>[2x]SNAACSKTNQNSKIATMKGDTITVADFYNEVKNSTASKQAVLSLLVSKVFEKQYGDKVSDKEVTKAYNEAAKYYGDSFSSALASRGYTKEDYKKQIRSEKLIEYAVKEEAKKEITDASYKSAYKDYKPEVTAQVIQLDSEDKAKSVLEEAKADGADFAKIAKDNTKGDKTEYSFDSGSTNLPSQVLSAALNLDKDGVSDVIKASDSTTYKPVYYIVKITKKTDKNADWKAYKKRLKEIIVSQKLNDSNFRNAVIGKAFKKANVKIKDKAFSEILSQY

Here, we solved the protein structures of two secreted parvulin and two secreted cyclophilin-like peptidyl-prolyl isomerase (PPIase) ATP-independent chaperones found in gram-positive streptococcal species. Two types of ATP-independent extracellular PPIases exist in pathogenic streptococci: the parvulin and cyclophilin families. Unlike cytoplasmic PPIases, extracellular PPIases have canonical secretion signal peptides that allow for their translocation across the cell membrane via the Sec pathway. These chaperones are lipidated to the outer leaflet of the membrane and function in the space between the bacterial membrane and cell wall.

Other streptococcal-secreted PPIases, such as S. mutans PrsA (SmuPrsA), are required for cell wall and membrane integrity and virulence in an infective endocarditis model. Additionally, the secretion of mutacin, the major factor in the colonization and establishment of S. mutans dental biofilms, is dependent on SmuPrsA. As key streptococcal virulence factors are dependent on PrsA for activity, we began characterizing streptococcal PrsA by determining the X-ray crystal structures of PrsA from S. pneumoniae and S. mutans. The SpnPrsA and SmuPrsA structures were solved to a resolution of 2.55 Å and 3.15 Å, respectively. As expected, SpnPrsA and SmuPrsA align well with an r.m.s.d. of 2.36 Å across 264 Cα atoms that share 49% sequence identity. Consistent with PrsA homologs, both streptococcal PrsA proteins have a central parvulin PPIase domain (SpnPrsA residues 143–241) linked to a foldase domain (N- and C-terminal regions). Furthermore, the streptococcal PrsA protomers are linked by a domain swap; protomers A and D each donate a segment of α1 and the β1, β2, and β7 strands to the domain swap. The interprotomer, three-stranded β-sheets formed by β1, β2, and β7 strands are presumed to interact with the cell membrane. Previous work of L. monocytogenes PrsA homologs has shown that dimerization is critical for PrsA function. This is consistent with our dimeric SmuPrsA structure, as is the dimer of dimers observed in the SpnPrsA structure.>MSGADRSPNAGAAPDSAPGQAAVASAYQRFEPRAYLRNNYAPPRGDLCNPNGVGPWKLRCLAQTFATGEVSGRTLIDIGSGPTVYQLLSACSHFEDITMTDFLEVNRQELGRWLQEEPGAFNWSMYSQHACLIEGKGECWQDKERQLRARVKRVLPIDVHQPQPLGAGSPAPLPADALVSAFCLQAVSPDLASFQRALDHITTLLRPGGHLL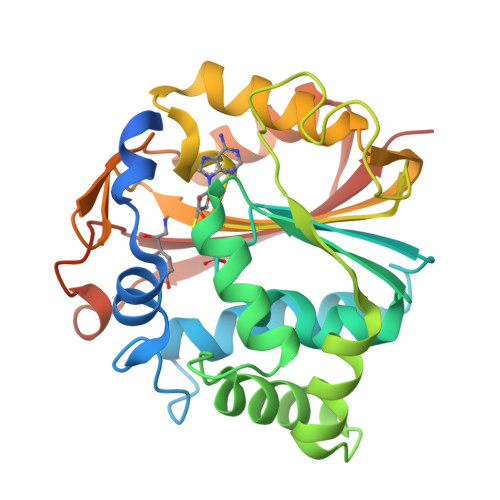LIGALEESWYLAGEARLTVVPVSEEEVREALVRSGYKVRDLRTYIMPAHLQTGVDDVKGVFFAWAQKVGLEHHHHHH[2x]> PAA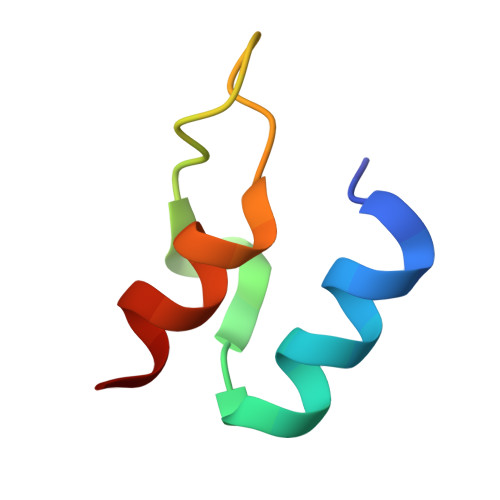PSIRRLARELGVDLTRLRGTGLAGRITEEDVRRAAGL methyl 2-acetamido-2-deoxy-alpha-D-galactopyranoside 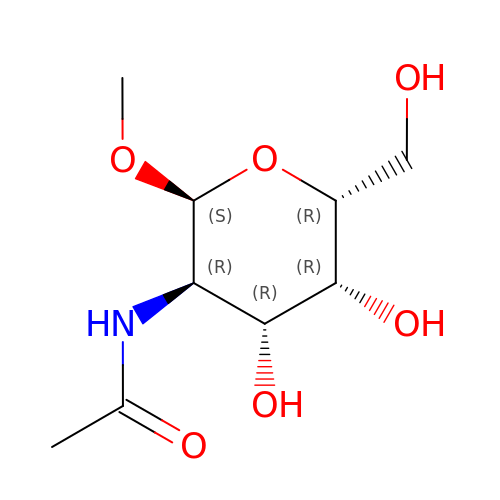| C9 H17 N O6 | ZEVOCXOZYFLVKN-ZEBDFXRSSA-N> MNPIHDRTSDYHKYLKVKQGDSDLFKLTVSDKRYIWYNPDPKERDSYECGEIVSETSDSFT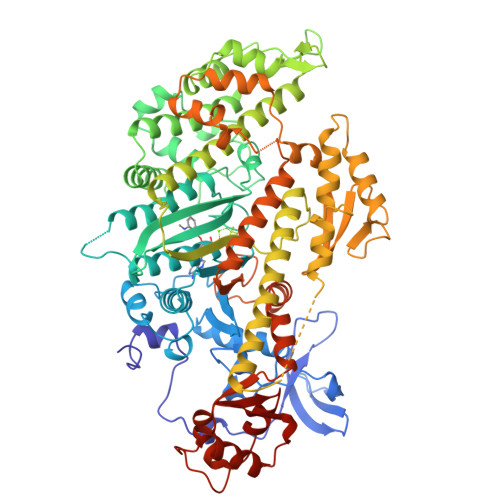FKTSDGQDRQVKKDDANQRNPIKFDGVEDMSELSYLNEPAVFHNLRVRYNQDLIYTYSGLFLVAVNPFKRIPIYTQEMVDIFKGRRRNEVAPHIFAISDVAYRSMLDDRQNQSLLITGESGAGKTENTKKVIQYLASVAGRNQANGSGVLEQQILQANPILEAFGNAKTTRNNNSSRFGKFIEIQFNNAGFISGASIQSYLLEKSRVVFQSTSERNYHIFYQLLAGATAEEKKALHLAGPESFNYLNQSGCVDIKGVSDEDEFKITRQAMDIVGFSQEEQMSIFKIIAGILHLGNIKFEKGAGEGAVLKDKTALNAASTVFGVNPSVLEKALMEPRILAGRDLVAQHLNVEKSSSSRDALVKALYGRLFLWLVKKINNVLCSERKAYFIGVLDISGFEIFKVNSFEQLCINYTNEKLQQFFNHHMFKVEQEKYLKEKINWTFIDFGLDSQATIDLIDGRQPPGILALLDEQSVFPNATDNTLITKLHSHFSKKNAKYEEPRFSKTEFGVTHYAGQVMYEIQDWLEKNKDPLQQDLELCFKDSSDNVVTKLFNDPNIASRAKKGANFLTVAAQYKEQLASLMATLETTNPHFVRCIIPNNKQLPAKLEDKVVLDQLRCNGVLEGIRITRKGFPNRIIYADFVKRYYDLAPNVPRDAEDSQKATDAVLKHLNIDPEQFRFGITKIFFRAGQLARIEEARELPN>[4x]HPETLVKVKDAEDQLGARVGYIELDLNSGKILESFRPEERFPMMSTFKVLLCGAVLSRVDAGQEQLGRRIHYSQNDLVEYSPVTEKHLTDGMTVRELCSAAITMSDNTAANLLLTTIGGPKELTAFLHNMGDHVTRLDRWEPELNEAIPNDER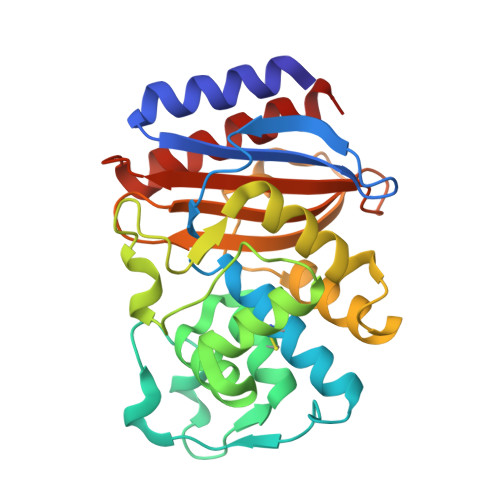DTTTPAAMATTLRKLLTGELLTLASRQQLIDWMEADKVAGPLLRSALPAGWFIADKSGAGERGSRGIIAALGPDGKPSRIVVNYTTGSQATMDERNRQIAEIGASLIKHW> ARTEKIYIYGASGHGLVCEDVAKNMGYKECIFLDDFKGMKFESTLPKYDFFIAIGNNEIRKKIYQKISENGFKIVNLIHKSALISPSA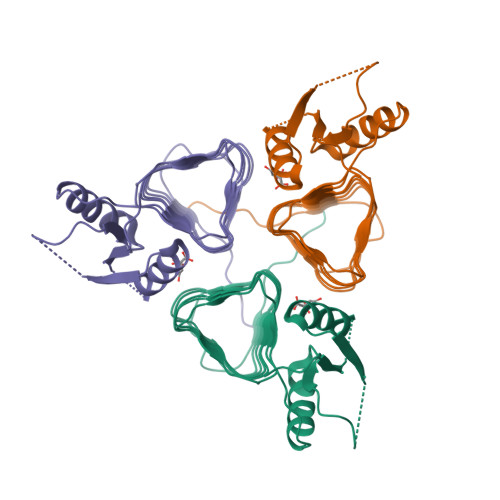IVEENAGILIMPYVVINAKAKIEKGVILNTSSVIEHECVIGEFSHVSVGAKCAGNVKIGKNCFLGINSCVLPNLSLADDSILGGGATLVKNQDEKGVFVGVPAKRM> MKVVKEFSVCGGRLIKLSHNSNSTKTSMNVNIYLPKHYYAQDFPRNKRIPTVFYLSGLTCTPDNASEKAFWQFQADKYGFAIVFPDTSPRGDEVANDPEGSWDFGQGAGFYLNATQEPYAQHYQMY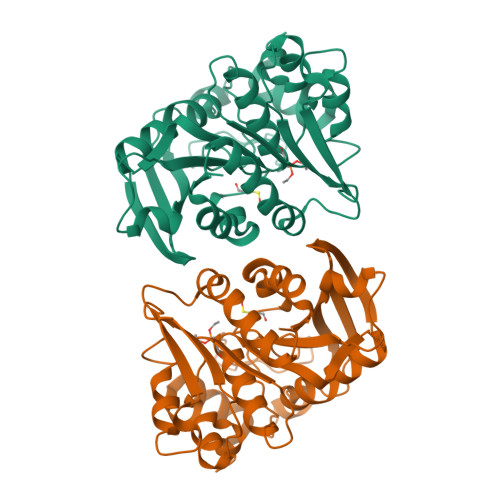DYIHKELPQTLDSHFNKNGDVKLDFLDNVAITGHSMGGYGAICGYLKGYSGKRYKSCSAFAPIVNPSNVPIGQKAFKGYLGEEKAQWEAYDPCLLIKNIRHVGDDRILIHVGDSDPFLEEHLKPELLLEAVKATSWQDYVEIKKVHGFDHSYYFVSTFVPEHAEFHARNLGLI> GACF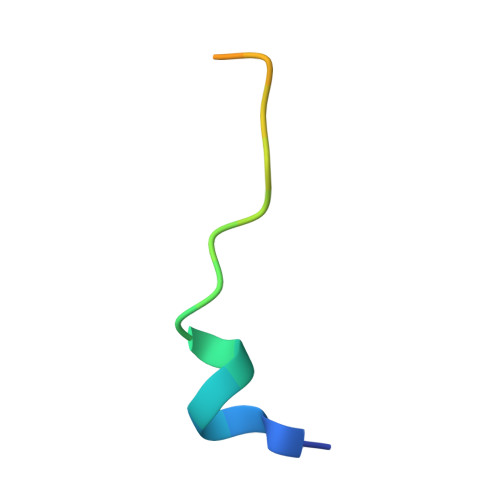KDAEYIYPSLESDDDDPA> MTQPLVGKQIL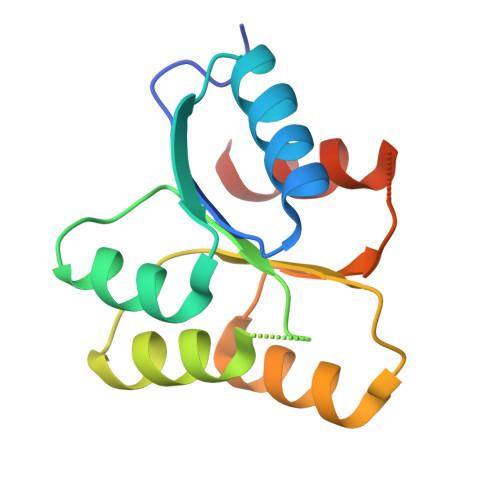IVEDEQVFRSLLDSWFSSLGATTVLAADGVDALELLGGFTPDLMICDIAMPRMNGLKLLEHIRNRGDQTPVLVISATENMADIAKALRLGVEDVLLKPVKDLNRLREMVFACLYPSMFN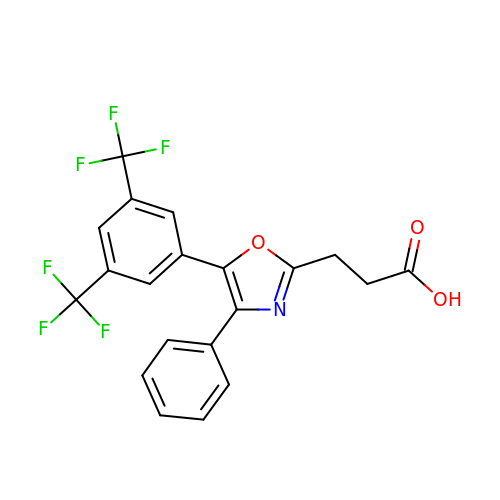3-(5-(3,5-bis(trifluoromethyl)phenyl)-4-phenyloxazol-2-yl)propanoic acid | C20 H13 F6 N O3 | KMMWBOHSOIDNLP-UHFFFAOYSA-N>[60x]GDWHCDTKWMGDHVITKSTRTWVLPTYGNHLYGPINFDGTTGSGANAAYAGYKTPWGYFDFNRFHCHFSPRDWQRLINNHTGIRPKGLKIKVFNVQVKEVTTQDSTKTIANNLTSTV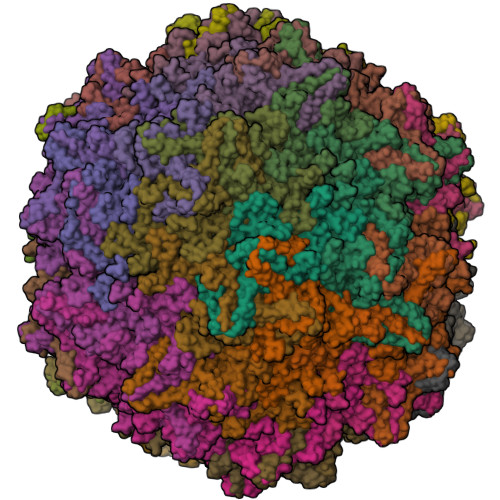QIFADENYDLPYVLGSATQGTFPPFPNDVFMLPQYAYCTLQGNSGKFVDRSAFYCLEYFPSQMLRTGNNFEFQFKFEEVPFHSGWAQSQSLDRLMNPLLDQYLIGDYGTDASGNLIYHRAGPNDLNEFYKNWAPAPYECIQNINSSDNTKNANSINGSNSTNKWGLQGRQAWDAPGFVQASTYEGAAAGQSLLNGVLTFDKSSATTSSPAATAVNRTIEDEIQGTNNFGNARNNIVAINQQTKGTNPTTGSTSQFETMPGMVWSNRDIYLQGPIWAKIPNTDGHFHPSPRMGGFGLKHPPPMILIKNTPVPADPPTTFNPMPQTSFITEYSTGQVTVEMLWEVQKESSKRWNPEVQFTSNFGTSDPAVDGIPFGINNLGTYVESRPIGTRYISKHL>GSKPRGKMSSYAFFVQTCREEHKKKHPDASVNFSEFSKKCSERWKTMSAKEKGKFEDMAKADKARYEREMKTYIPP[2x]

High-mobility group protein 1 (HMGB1) is an essential and ubiquitous DNA architectural factor that influences a myriad of cellular processes. HMGB1 contains two DNA-binding domains, box A and box B, which have little sequence specificity but have remarkable abilities to underwind and bend DNA. The HMG box is the defining and characteristic domain of the HMGB family. This domain comprises three α-helices with an L-shaped structure, in which helix I and II form a short arm and helix III together with an N-terminal stretch of amino acids forms a long arm. HMGB1 box A is an exception because Ala16 at the 1° site cannot intercalate DNA but Phe37 at the 2° site can, and this is thought to be responsible for the superior ability of box A to recognize pre-bent DNA.

The refined model at a resolution of 2.0 Å was well resolved, with an asymmetric unit comprising one unbound straight DNA duplex and one bent DNA duplex bound by two box A domains. These duplexes form a pseudo-continuous helix throughout the crystal. The structure also contains a single hexahydrated magnesium ion and a network of water molecules. The two box A domains bind in an approximately symmetric manner about the dyad axis of the palindromic DNA decamer, with water-mediated interactions between the domains. Two box A domains of HMGB1 collaborate in an unusual configuration in which the Phe37 residues of both domains stack together and intercalate the same CG base pair, generating highly kinked DNA. The two phenyl rings of Phe37 are parallel to each other at 3.5 Å, a distance indicative of π-stacking. Thus, this collaborative binding mode, whereby the 2° intercalation residues of two HMG box A domains act in the same base step, has not previously been observed. At the kink in the box A–DNA structure, the minor groove widens, the major groove narrows and the DNA is underwound; in particular, the C5G6/C15G16 base step has a roll angle of 74.85°, a twist angle of 4.82° and a rise of 6.64 Å, compared with standard values of a roll of 0.60°, a twist of 36.00° and a rise of 3.32 Å for B-DNA. Thus, the collaborative binding of both box A domains distorts DNA similarly to cisplatin alone.> PAGIIPTGNVLSTIEVCAHRCIFDFFKQIRSDDNSLYSAQFDILLGTYCNTLNFVRFLELGLSVACICTKFPELAYVRDGVIQFEVQQPMIARDGPHPVDQPVHNYMVKRIHKRSLSAAFAIASEALSLLSNTYVDGTEIDSSLRIRAIQQMARNLRTVLDSFERGTADQLLGVLLEKAPPLSLLSPINKFQPEGHLNRVARAALLSDLKRRVCADMFFMTRHAREPRLISAYLSDMVSCTQPSVMVSRITHTNTRGRQVDGVLVTTATLKRQLLQGILQIDDTAADVPVTYGEMVLQGTNLVTALVMGKAVRGMDDVARHLLDITDPNTLNIPSIPPQSNSDSTTAGLPVNARVPADLVIVGDKLVFLEALERRVYQATRVAYPLIGNIDITFIMPMGVFQANSMDRYTRHAGDFSTVSEQDPRQFPPQGIFFYNKDGILTQLTLRDAMGTICHSSLLDVEATLVALRQQHLDRQCYFGVYVAEGTEDTLDVQMGRFMETWADMMPHHPHWVNEHLTILQFIAPSNPRLRFELNPAFDFFVAPGDVDLPGPQRPPEAMPTVNATLRIINGNIPVPLCPISFRDCRGTQLGLGRHTMTPATIKAVKDTFEDRAYPTIFYMLEAVIHGNERNFCALLRLLTQCIRGYWEQSHRVAFVNNFHMLMYITTYLGNGELPEVCINIYRDLLQHVRALRQTITDFTIQGEGHNGETSEALNNILTDDTFIAPILWDCDALIYRDEAARDRLPAIRVSGRNGYQALHFVDMAGHNFQRRDNVLIHGRPVRGDTGQAIPITPHHDREWGILSKIYYYIVIPAFSRGSCCTMGVRYDRLYPALQAVIVPEIPADEEAPTTPEDPRHPLHAHQLVPNSLNVYFHNAHLTVDGDALLTLQELMGDMAERTTAILVSSAPDAGAATATTRNMRIYDGALYHGLIMMAYQAYDETIATGTFFYPVPVNPLFACPEHLASLRGMTNARRVLAKMVPPIPPFLGANHHATIRQPVAYHVTHSKSDFNTLTYSLLGGYFKFTPISLTHQLRTGFHPGIAFTVVRQDRFATEQLLYAERASESYFVGQIQVHHHDAIGGVNFTLTQPRAHVDLGVGYTAVCATAALRCPLTDMGNTAQNLFFSRGGVPMLHDNVTESLRRITASGGRLNPTEPLPIFGGLRPATSAGIARGQASVCEFVAMPVSTDLQYFRTACNPRGRASGMLYMGDRDADIEAIMFDHTQSDVAYTDRATLNPWASQKHSYGDRLYNGTYNLTGASPIYSPCFKFFTPAEVNTNCNTLDRLLMEAKAVASQSSTDTEYQFKRPPGSTEMTQDPCGLFQEAYPPLCSSDAAMLRTAHAGETGADEVH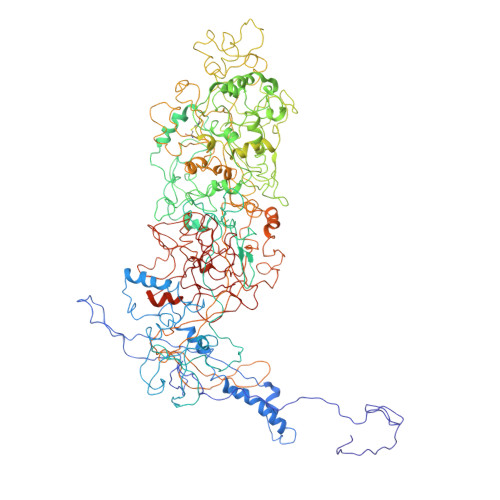LAQYLIRDASPLRGCLPL> MKLERVTVKNFRSHSDTVVEFKEGINLIIGQNGSGKSSLL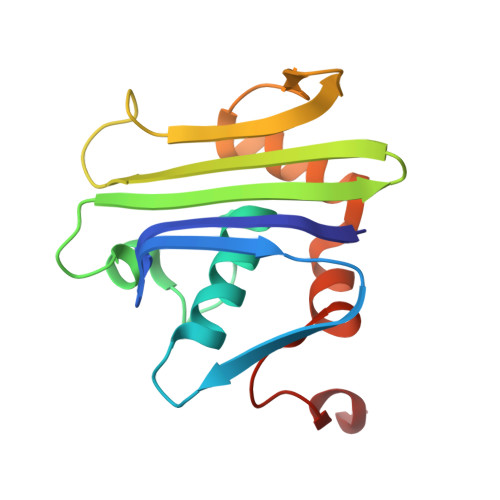DAILVGLYWPLRIKDIKKDEFTKVGARDTYIDLIFEKDGTKYRITRRFLKGYSSGEIHAMKRLVGNEWKHVTEPSSKAISAFMEKLIPYNIFLNAIYIRQGQIDAILES>[2x]MGPVWRKHYITYRINNYTPDMNREDVDYAIRKAFQVWSNVTPLKFSKINTGMADILVVFARGAHGDFHAFDGKGGILAHAFGPGSGIGGDAHFDED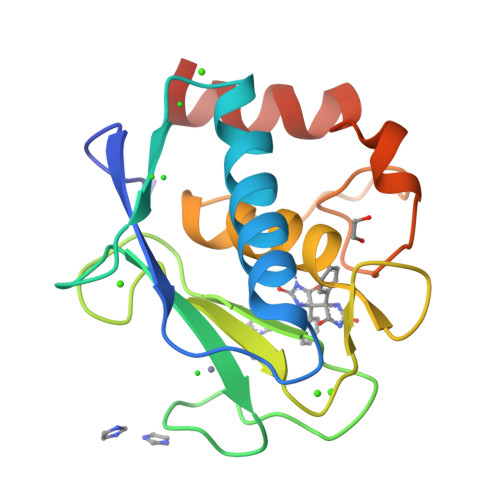EFWTTHSGGTNLFLTAVHAIGHSLGLGHSSDPKAVMFPTYKYVDINTFRLSADDIRGIQSLYGHHHHH>XFAAAVGLAAPQVP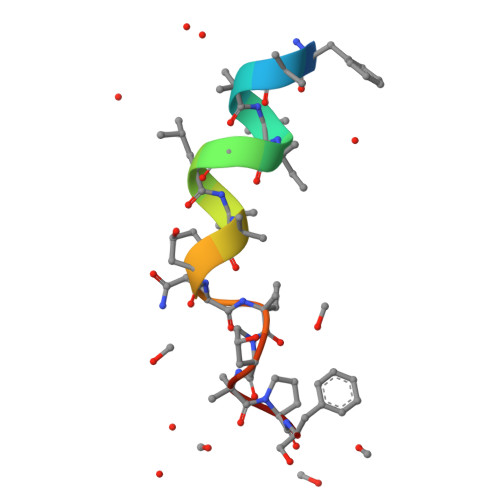APF[2x]> MMQSAMCIPLWPARNGNTAHLVMCPFAGGSSSAFRHWQAEQLADCALSLVTWPGRDRLRHLEPLRSITQLAALLANELEASVSPDTPLLLAGHSMGAQVAFETCRLLEQRGLAPQGLIISGCHAPHLHSERQLSHRDDADFIAELIDIGGCSPELRENQ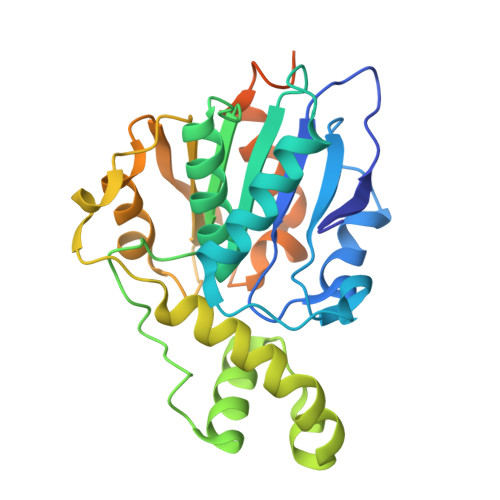ELMSLFLPLLRADFYATESYHYDSPDVCPPLRTPALLLCGSHDREASWQQVDAWRQWLSHVTGPVVIDGDHFYPIQQARSFFTQIVRHFPHAFSAMTAWQKQPSTSERKLGPEQKLISEEDLNSAVDHHHHHH>MLSRKGIIPEEYVLTRLAEDPAEPRYRTRERRARFVSKKGNCNVAHKNIREQGRFLQDVFTTLVDLKWPHTLLIFTMSFLCSWLLFAMVWWLIAFAHGDLAPGEGTNVPCVTSIHSFSSAFLFSIEVQVTIGFGGRMVTEECPLAILILIVQNIVGLMINAIMLGCIFMKTAQAKRRAETLIFSKHAVITLRHGRLCFMLRVGDLRKSMIISATIHMQVVRKTTSPEGEVVPLHQVDIPMENGVGGNGIFLVAPLIIYHVIDSNSPLYDLAPSDLHHHQDLEIIVILEGVVETTGITTQARTSYLADEILWGQRFVPIVAEEDGRYSVDYSKFGNTIKVPTPLCTARQLDEDRSLLDALTLASSRGPLRKRSVAVAKAKPKFSISPDSLS[4x];>[4x]MPLAFCGTENHSAAYRVDQGVLNNGCFVDALNVVPHVFLLFITFPILFIGWGSQSSKVHIHHSTWLHFPGHNLRWILTFILLFVLVCEIAEGILSDGVTESRHLHLYMPAGMAFMAAITSVVYYHNIETSNFPKLLIALLIYWTLAFITKTIKFVKFYDHAIGFSQLRFCLTGLLVILYGMLLLVEVNVIRVRRYIFFKTPREVKPPEDLQDLGVRFLQPFVNLLSKGTYWWMNAFIKTAHKKPIDLRAIGKLPIAMRALTNYQRLCVAFDAQARKDTQSPQGARAIWRALCHAFGRRLILSSTFRILADLLGFAGPLCIFGIVDHLGKENHVFQPKTQFLGVYFVSSQEFLGNAYVLAVLLFLALLLQRTFLQASYYVAIETGINLRGAIQTKIYNKIMHLSTSNLSMGEMTAGQICNLVAIDTNQLMWFFFLCPNLWAMPVQIIVGVILLYYILGVSALIGAAVIILLAPVQYFVATKLSQAQRSTLEHSNERLKQTNEMLRGMKLLKLYAWESIFCSRVEVTRRKEMTSLRAFAVYTSISIFMNTAIPIAAVLITFVGHVSFFKESDLSPSVAFASLSLFHILVTPLFLLSSVVRSTVKALVSVQKLSEFLSSAEIREEQCAPREPAPQGQAGKYQAVPLKVVNRKRPAREEVRDLLGPLQRLAPSMDGDADNFCVQIIGGFFTWTPDGIPTLSNITIRIPRGQLTMIVGQVGCGKSSLLLATLGEMQKVSGAVFWNSNLPDSEGEDPSSPERETAAGSDIRSRGPVAYASQKPWLLNATVEENITFESPFNKQRYKMVIEACSLQPDIDIL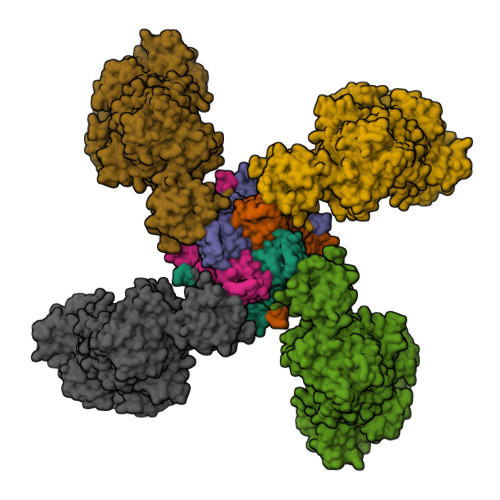PHGDQTQIGERGINLSGGQRQRISVARALYQQTNVVFLDDPFSALDVHLSDHLMQAGILELLRDDKRTVVLVTHKLQYLPHADWIIAMKDGTIQREGTLKDFQRSECQLFEHWKTLMNRQDQELEKETVMERKASEPSQGLPRAMSSRDGLLLDEEEEEEEAAESEEDDNLSSVLHQRAKIPWRACTKYLSSAGILLLSLLVFSQLLKHMVLVAIDYWLAKWTDSALVLSPAARNCSLSQECDLDQSVYAMVFTLLCSLGIVLCLVTSVTVEWTGLKVAKRLHRSLLNRIILAPMRFFETTPLGSILNRFSSDCNTIDQHIPSTLECLSRSTLLCVSALTVISYVTPVFLVALLPLAVVCYFIQKYFRVASRDLQQLDDTTQLPLLSHFAETVEGLTTIRAFRYEARFQQKLLEYTDSNNIASLFLTAANRWLEVRMEYIGACVVLIAAATSISNSLHRELSAGLVGLGLTYALMVSNYLNWMVRNLADMEIQLGAVKRIHALLKTEAESYEGLLAPSLIPKNWPDQGKIQIQNLSVRYDSSLKPVLKHVNALISPGQKIGICGRTGSGKSSFSLAFFRMVDMFEGRIIIDGIDIAKLPLHTLRSRLSIILQDPVLFSGTIRFNLDPEKKCSDSTLWEALEIAQLKLVVKALPGGLDAIITEGGENFSQGQRQLFCLARAFVRKTSIFIMDEATASIDMATENILQKVVMTAFADRTVVTIAHRVHTILSADLVMVLKRGAILEFDKPETLLSQKDSVFASFVRADK>GUACGAAGGAAGGUUUGGUAUGUGGUAUAUUCGU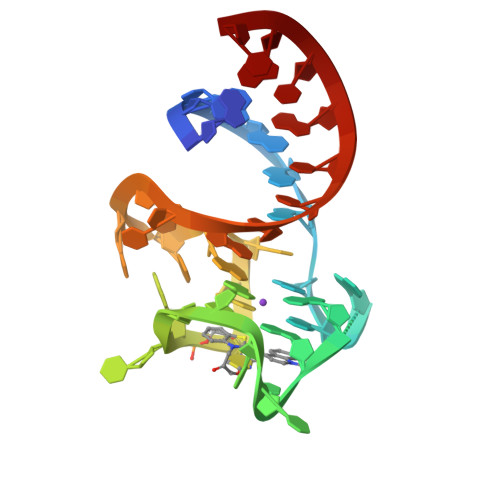AC[4x]> SAVKAARYGKDNVRVYKVHKDEKTGVQTVYEMTVCVLLEGEIETSYTKA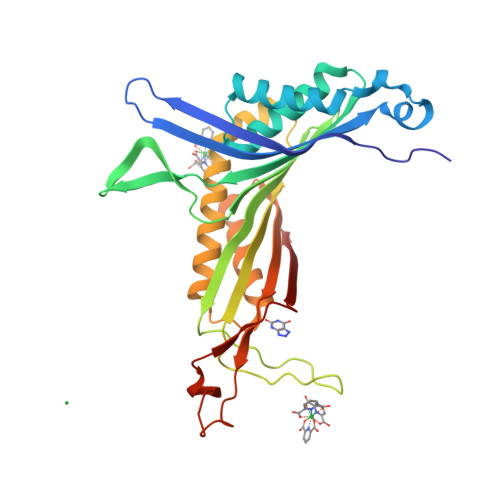DNSVIVATDSIKNTIYITAKQNPVTPPELFGSILGTHFIEKYNHIHAAHVNIVCHRWTRMDIDGKPHPHSFIRDSEEKRNVQVDVVEGKGIDIKSSLSGLTVLKSTNSQFWGFLRDEYTTLKETWDRILSTDVDATWQWKNFSGLQEVRSHVPKFDATWATAREVTLKTFAEDNSASVQATMYKMAEQILARQQLIETVEYSLPNKHYFEIDLSWHKGLQNTGKNAEVFAPQSDPNGLIKCTVGRS>[4x]GMSSLPAVYIVSSARTPVGSFLGSLSSLTAPQLGAHAIKAALAKVDGLKPSDVQEVFFGNVISANVGQNPARQCALGAGLEESTICTTVN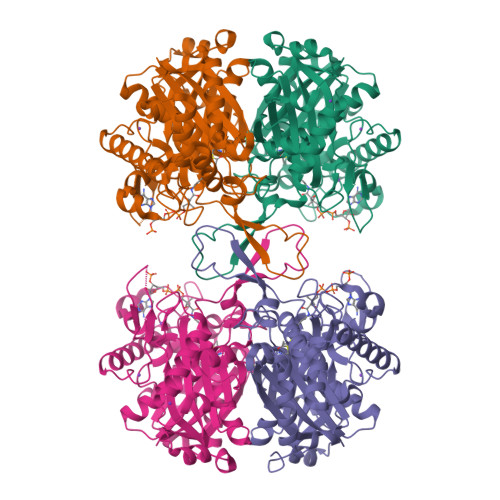KVCASGLKAIILGAQTIMTGNADVVVAGGTESMSNAPHYLPNLRTGAKYGHQSLVDGIMKDGLTDAGKQELMGLQAEECAQDHGFSREQQDEYAIRTYEKAQAAQKAGLFDEEIAPIQLPGFRGKPDVTVTQDEEPKNLNPEKLRAIKPAFIPGSGTVTAPNSSPLNDGAAAVVLVSEAKLKELNLKPVAKILGWGDAAQQPSKFTTAPALAIPKALKHAGVGQDAIDAFEINEAFSVVALANMKLLGIPEEKVNLHGGAVAIGHPIGASGARILTTLLGVLKAKKGKLGCAGICNGGGGASALVVELL>MADVFHLGLTKAMLDGATLAIVPGDPERVKRIAELMDNATFLASHREYTSYLAYADGKPVVICSTGIGGPSTSIAVEELAQLGVNTFLRVGTTGAIQPHVNVGDVIVTQASVRLDGASLHFAPMEFPAVANFECTTAMVAACRDAGVEPHIGVTASSDTFYPGQERYDTVTGRVTRRFAGSMKEWQDMGVLNYEMESATLFTMCATQGWRAACVAGVIV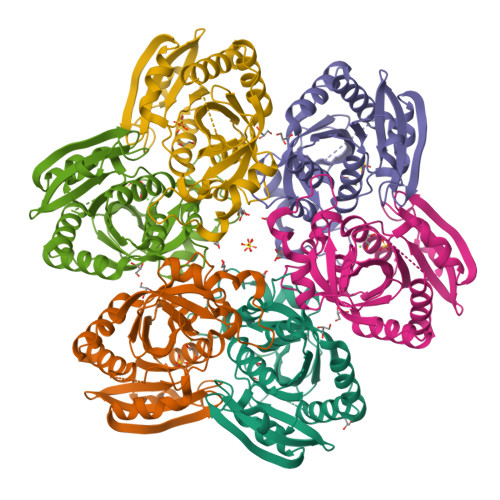NRTQQEIPDEATMKKTEVSAVSIVVAAAKKLLA[6x]> MPEIVDTCSLASPASVCRTKHLHLRCSVDFTRRTLTGTAALTVQSQEDNLRSLVLDTKDLTIEKVVINGQEVKYALGERQSYKGSPMEISLPIALSKNQEIVIEISFETSPKSSALQWLTPEQTSGKEHPYLFSQCQAIHCRAILPCQDTPSVKLTYTAEVSVPKELVALMSAIRDGETPDPEDPSRKIYKFIQKVPIPCYLIALVVGALESRQIGPRTLVWSEKEQVEKSAYEFSETESMLK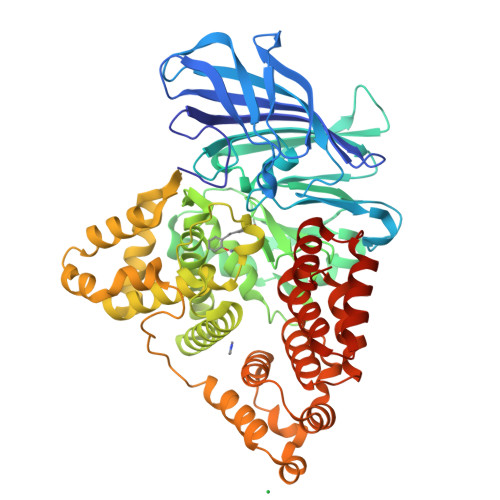IAEDLGGPYVWGQYDLLVLPPSFPYGGMENPCLTFVTPTLLAGDKSLSNVIAHEISHSWTGNLVTNKTWDHFWLNEGHTVYLERHICGRLFGEKFRHFNALGGWGELQNSVKTFGETHPFTKLVVDLTDIDPDVAYSSVPYEKGFALLFYLEQLLGGPEIFLGFLKAYVEKFSYKSITTDDWKDFLYSYFKDKVDVLNQVDWNAWLYSPGLPPIKPNYDMTLTNACIALSQRWITAKEDDLNSFNATDLKDLSSHQLNEFLAQTLQRAPLPLGHIKRMQEVYNFNAINNSEIRFRWLRLCIQSKWEDAIPLALKMATEQGRMKFTRPLFKDLAAFDKSHDQAVRTYQEHKASMHPVTAMLVGKDLKVDVDHHHHHH One extracellular protein family that arose through domain replication and gene duplication is the gel-forming mucins, huge glycoproteins that coat and protect the epithelia in the lungs, intestines, and other organs. A remarkable variation on the theme of mucins arose with the evolution of the complex vasculature in the vertebrate lineage. von Willebrand factor (VWF), a glycoprotein responsible for hemostasis, has a similar domain organization and is homologous to mucins in its amino- and carboxyl-terminal regions. Under acidic conditions, the amino termini of mucins and VWF form noncovalent intermolecular interactions that juxtapose VWD3 assemblies from different CTCK-linked dimers. We present residue-resolution structures of VWF and MUC2 amino-terminal segment tubules, enabling comparison between them and an analysis of the features that stabilize each one.

We subsequently discovered using dynamic light scattering (DLS) that a dimeric MUC2 amino-terminal fragment spanning the D1D2D3 region but lacking CysD1 could also self-assemble, but only at a lower pH. Remarkably, in TEM samples prepared at pH 5.4, the D1D2D3 fragment exhibited tubules that resembled the VWF tubules found in WPBs, both with diameters of ∼25 nm. The VWF and MUC2 tubules also both display twofold symmetry perpendicular to the helix axis. They differ, however, in that the VWF tubule is a one-start helix, whereas the MUC2 tubule is a two-start helix. The MUC2 tubule has a helical twist of ∼83.2° (about 4.3 subunits per turn) and an axial rise of ∼6.95 nm per subunit. Due to the larger axial rise of the two-start compared to the one-start helix, a helical turn of MUC2 (its lead) extends almost 30 nm along the helix axis, whereas a turn of VWF extends only about 12 nm. The MUC2 and VWF tubule maps indicated contacts between one helical layer and the next, which in MUC2 are made between the two separate, intertwined helices. The MUC2 helix map showed additional interturn contacts not seen in VWF. In the MUC2 tubule, C8-1 modules from each bead contact one another, with an interface area of less than 200 Å2. The MUC2 tubule also has a second contact between helical turns (gray arrows). The MUC2 tubule thus appears to be stabilized mainly by quaternary interactions between turns of the helix, whereas the more rigid packing of the bridge in VWF appears to dictate the geometry of its tubule.

>SELQTEGRTRNHGHNVCSTWGNFHYKTFDGDVFRFPGLCDYNFASDCRGSYKEFAVHLKRGPGQAEAPAGVESILLTIKDDTIYLTRHLAVLNGAVVSTPHYSPGLLIEKSDAYTKVYSRAGLTLMWNREDALMLELDTKFRNHTCGLCGDYNGLQSYSEFLSDGVLFSPLEFGNMQKINQPDVVCEDPEEEVAPASCSEHRAECERLLTAEAFADCQDLVPLEPYLRACQQDRCRCPGGDTCVCSTVAEFSRQCSHAGGRPGNWRTATLCPKTCPGNLVYLESGSPCMDTCSHLEVSSLCEEHRMDGCFCPEGTVYDDIGDSGCVPVSQCHCRLHGHLYTPGQEITNDCEQCVCNAGRWVCKDLPCPGTCALEGGSHITTFDGKTYTFHGDCYYVLAKGDHNDSYALLGELAPCGSTDKQTCLKTVVLLADKKKNVVVFKSDGSVLLNELQVNLPHVTASFSVFRPSSYHIMVSMAIGVRLQVQLAPVMQLFVTLDQASQGQVQGLCGNFNGLEGDDFKTASGLVEATGAGFANTWKAQSSCHDKLDWLDDPCSLNIESANYAEHWCSLLKKTETPFGRCHSAVDPAEYYKRCKYDTCNCQNNEDCLCAALSSYARACTAKGVMLWGWREHVCNKDVGSCPNSQVFLYNLTTCQQTCRSLSEADSHCLEGFAPVDGCGCPDHTFLDEKGRCVPLAKCSCYHRGLYLEAGDVVVRQEERCVCRDGRLHCRQIRLIGQSCTAPKIHMDCSNLTALATSKPRALSCQTLAAGYYHTECVSGCVCPDGLMDDGRGGCVVEKECPCVHNNDLYSSGAKIKVDCNTCTCKRGRWVCTQAVCHGTCSIYGSGHYITFDGKYYDFDGHCSYVAVQDYCGQNSSLGSFSIITENVPCGTTGVTCSKAIKIFMGRTELKLEDKHRVVIQRDEGHHVAYTTREVGQYLVVESSTGIIVIWDKRTTVFIKLAPSYKGTVCGLCGNFDHRSNNDFTTRDHMVVSSELDFGNSWKEAPTCPDVSTNPEPCSLNPHRRSWAEKQCSILKSSVFSICHSKVDPKPFYEACVHDSCSCDTGGDCECFCSAVASYAQECTKEGACVFWRTPDLCPIFCDYYNPPHECEWHYEPCGNRSFETCRTINGIHSNISVSYLEGCYPRCPKDRPIYEEDLKKCVTADKCGCYVEDTHYPPGASVPTEETCKSCVCTNSSQVVCRPEEGKILNQTQDGAFCYWEICGPNGTVEKHFNICSITHHHHHH[6x]>MLSPEALTTAVDAAQQAIALADTLDVLARVKTEHLGDRSPLALARQALAVLPKEQRAEAGKRVNAARNAAQRSYDERLATLRAERDAAVLVAEGIDVTLPSTRVPAGARHPIIMLAEHVADTFIAMGWELAEGPEVETEQFNFDALNFPADHPARGEQDTFYIAPEDSRQLLRTHTSPVQIRTLLARELPVYIISIGRTFRTDELDATHTPIFHQVEGLAVDRGLSMAHLRGTLDAFARAEFGPSARTRIRPHFFPFTEPSAEVDVWFANKIGGAAWVEW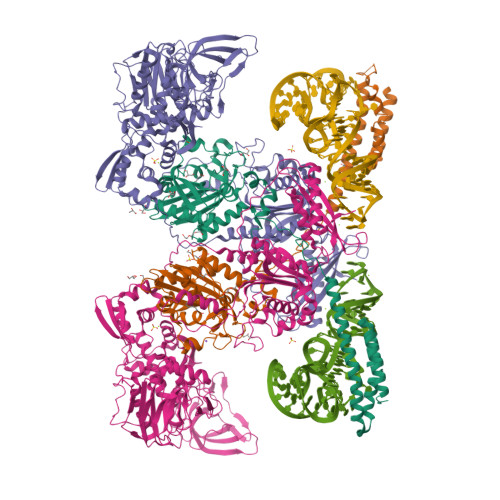GGCGMVHPNVLRATGIDPDLYSGFAFGMGLERTLQFRNGIPDMRDMVEGDVRFSLPFGVGA[2x];>[2x]QSNAMRLPYSWLREVVAVGASGWDVTPGELEQTLLRIGHEVEEVIPLGPVDGPVTVGRVADIEELTGYKKPIRACAVDIGDRQYREIICGATNFAVGDLVVVALPGATLPGGFTISARKAYGRNSDGMICSAAELNLGADHSGILVLPPGAAEPGADGAGVLGLDDVVFHLAITPDRGYCMSVRGLARELACAYDLDFVDPASNSRVPPLPIEGPAWPLTVQPETGVRRFALRPVIGIDPAAVSPWWLQRRLLLCGIRATCPAVDVTNYVMLELGHPMHAHDRNRISGTLGVRFARSGETAVTLDGIERKLDTADVLIVDDAATAAIGGVMGAASTEVRADSTDVLLEAAIWDPAAVSRTQRRLHLPSEAARRYERTVDPAISVAALDRCARLLADIAGGEVSPTLTDWRGDPPCDDWSPPPIRMGVDVPDRIAGVAYPQGTTARRLAQIGAVVTHDGDTLTVTPPSWRPDLRQPADLVEEVLRLEGLEVIPSVLPPAPAGRGLTAGQQRRRTIGRSLALSGYVEILPTPFLPAGVFDLWGLEADDSRRMTTRVLNPLEADRPQLATTLLPALLEALVRNVSRGLVDVALFAIAQVVQPTEQTRGVGLIPVDRRPTDDEIAMLDASLPRQPQHVAAVLAGLREPRGPWGPGRPVEAADAFEAVRIIARASRVDVTLRPAQYLPWHPGRCAQVFVGESSVGHAGQLHPAVIERSGLPKGTCAVELNLDAIPCSAPLPAPRVSPYPAVFQDVSLVVAADIPAQAVADAVRAGAGDLLEDIALFDVFTGPQIGEHRKSLTFALRFRAPDRTLTEDDASAARDAAVQSAAERVGAVLRG> APLNAARPAEERAALLAWVKERLHEEYGDQDPTPRRDPMHELISTILSQRTTHADEEAAYQELRTLGDWDAITLAPT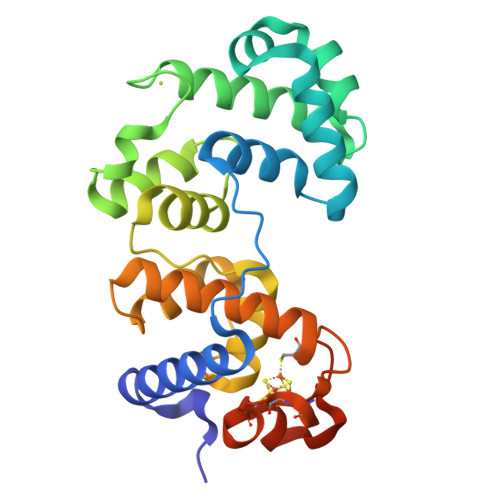DAVAHAIRRSNLPESKAPRIQETLRRIKAAPGGYDLDFLRDLPVKDALKWLTDLPGVGVKTASLVLLFNYARPVFPVDTHVHRVSTRVGVIPRMGEQAAHRALLALLPPDPPYLYELHINFLSHGRQVCTWTRPKCGKCILRERCDAYALYGDKVPSFSEKPVKGEKPAKG> MSSALTDLFPLPIVQAPMAGGVSVPQLAAAVCEAGGLGFLAAGYKTADGM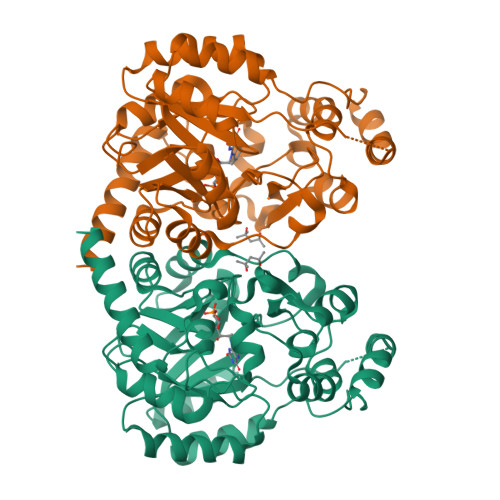YQEIKRLRGLTGRPFGVNVFMPQPELAESGAVEVYAHQLAGEAAWYETELGDPDGGRDDGYDAKLAVLLDDPVPVVSFHFGVPDREVIARLRRAGTLTLVTATTPEEARAVEAAGADAVIAQGVEAGGHQGTHRDSSEDDGAGIGLLSLLAQVREAVDIPVVAAGGIMRGGQIAAVLAAGADAAQLGTAFLATDESGAPGPHKRALTDPLFARTRLTRAFTGRPARSLVNRFLREHGPYAPAAYPDVHHLTSPLRKAAAKAGDAQGMALYAGQGHRMARELPAGRLVEVLAAELAEARTALSDASRENESRKGHHHHHH>[4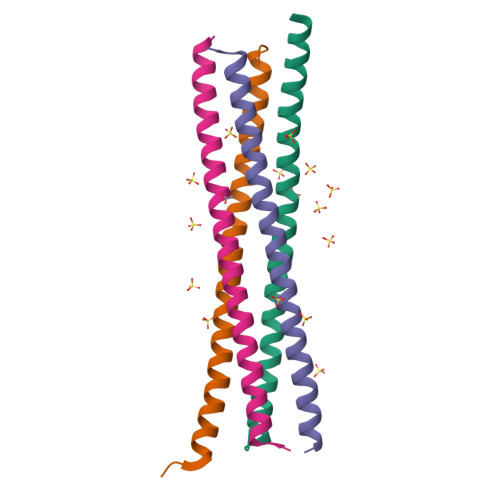x]SMDEECVLEAENKKLVEDQEKLKTELRKTSDALSKAQNDVMEMKMQSERLSKEYDQLLKEHSEL N-[(3S)-7-(2-cyclopropylethynyl)-5-methyl-4-oxidanylidene-2,3-dihydro-1,5-benzoxazepin-3-yl]-5-(phenylmethyl)-4H-1,2,4-triazole-3-carboxamide 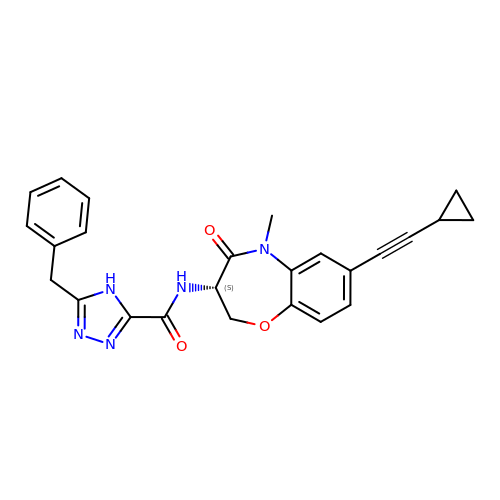| C25 H23 N5 O3 | QDIMLDKKJUQINI-IBGZPJMESA-N N-[3-(5-chloro-2-methoxyphenyl)-1-methyl-1H-pyrazol-4-yl]-1H-pyrazolo[4,3-c]pyridine-7-carboxamide | C18 H15 Cl N6 O2 | 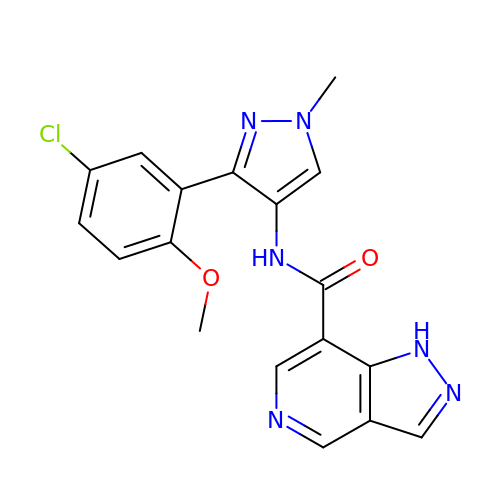NBFASNUBTMTAFQ-UHFFFAOYSA-N>MNPNQKIITIGSVSLIIATVCFLMQIAILVTTVTLHFKQHECDSPSSNQVMLCEPIIIERNITEIVYLNNTTIEKETCPKLVEYRNWSKPQCKITGFAPFSKDNSIRLSAGGDIWVTREPYVSCDPGKCYQFALGQGTTLDNKHSNDTIHDRIPHRTLLMNELGVPFHLGTRQVCIAWSSSSCHDGKAWLHVCVTGDDKNATASFIYDGRLVDSIGSWSQNILRTQESECVCINGTCTVVMTDGSASGRADTRILFIEEGKIVHISPLSGSAQHVEECSCYPRYPDVRCICRDNWKGSNRPIVDINMKDYSIDSSYVCSGLVGDTPRNDDRSSKSNCRNPNNERGNHGVKGWAFDNGNDVWMGRTISKDLRSGYETFKVIGGWSTPNSKSQINRQVIVDSDNRSGYSGIFSVEGKSCINRCFYVELIRGREQETRVWWTSNSIVVFCGTSGTYGTGSWPDGANINFMPI[4x]

Influenza A virus has two surface glycoproteins, hemagglutinin (HA) and neuraminidase (NA), that act as the major antigens. NA is a type II transmembrane protein that forms a homotetramer. The natural function of NA is to cleave the sialic acids from cellular receptors to facilitate virus release and from newly synthesized HA to prevent virion aggregation. Neuraminidase (NA) of human influenza H3N2 virus has evolved rapidly and been accumulating mutations for more than half-century.

To further examine the structural mechanism of epistasis between K385N and N387K, we determined the crystal structure of NAs from Bil69, SD93, and Mos99 to 1.54 Å, 1.65 Å, and 1.40 Å, respectively. K385N alone is unlikely to cause a change in backbone conformation, since Bil69 NA and Mos99 NA carry different amino acids at residue 385 and yet have the same backbone conformation in this region. Similarly, our result implies that the permissive mutations for N336H emerged between 1969 and 1971, since mutating residue 336 to His was neutral in Bil71 and Alb76 but reduced the virus titer of Bil69 to below the detection limit. Our virus rescue experiment further validated that N356D was a permissive mutation for N336H and was neutral when being introduced alone. Same as N336H, N336Y also reduced the titer of Bil69 to below the detection limit and the addition of N356D could restore it to the WT level. In contrast to N387K, N336H did not reduce the Tm of Bil69 NA. However, the first differential curve of the thermal shift assay for Bil69 N336H had an atypical shape. Similarly, the first differential curve for Bil69 N336Y showed two peaks. These results indicate the presence of multiple oligomeric states, hence protein aggregates. The shapes of their first differential curves returned to WT-like when N356D was introduced.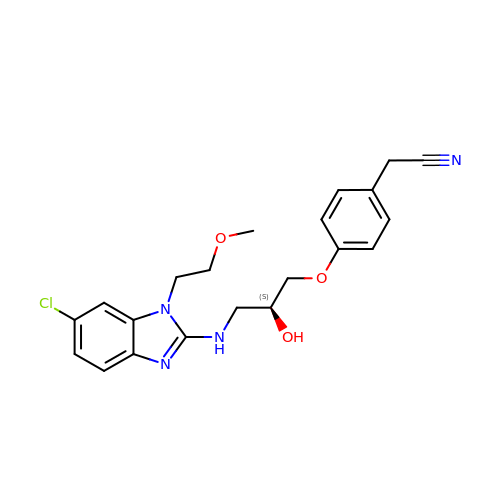2-[4-[(2~{S})-3-[[6-chloranyl-1-(2-methoxyethyl)benzimidazol-2-yl]amino]-2-oxidanyl-propoxy]phenyl]ethanenitrile | C21 H23 Cl N4 O3 | MZCRDZUXHLAMCH-KRWDZBQOSA-N>[3x]GSHMSYNNIPAGKDAPNDIYVIIEIPANAAPIKYEIDKDSDALFVDRFMGTAMFYPANYGYVPNTLSEDGDPLDVLVVTPYPVAAGSVIRCRPVGKLNMEDDGGIDAKLIAVPHEKLSPLYKDVKEYTDLPQLLINQVEHFFSHYKDLEPGRWVKISGWEGADVAKAEVIKAIEAAK

However, because PPi is stable under normal conditions, inorganic pyrophosphatase (PPase) has evolved to specifically hydrolysis the molecule. Here, we solved four crystal structures of a family I type PPase from a strain of the pathogen Acinetobacter baumannii. The crystal structures of AbPPase showed that the enzyme has a typical Rossman fold domain that is highly conserved compared to other PPases. Family I PPases are hexamers formed by two stacks of trimers.

The space group of Structure 4 (K149R) is P41212, with three monomers in the trimer of the asymmetric unit. Thus, it could form a hexamer with the trimer from another asymmetry unit. K149R showed a similar activity as WT AbPPase, indicating that the mutation of Lys149 to Arg had no influence on AbPPase activity. In addition, K149R could be co-crystallized with PPi, suggesting that substitution of Lys149 to Arg did not affect the affinity of AbPPase for PPi. Moreover, Lys149 in all the monomers displayed different conformations, and mutant K149R exhibited full hydrolytic activity indicates that this residue is not important for substrate binding and catalytic activity. In the catalytic center of K149R, M1, and M2 were not located at the same positions as M1 and M2 in the wild-type enzyme. But this variant still displayed almost the same catalytic activity as WT AbPPase. K149R was also sensitive to monovalent cation-induced inhibition like WT AbPPase. The positions of Lys30, Arg44, Tyr56, Asp71, Asp98, Asp103, Lys105, Tyr142, and Lys143 in WT and K149R are also relatively the same, indicating that the conformations of these residues are crucial for binding PPi-M3.>GSGDSGSPGIATPLVLGENLCSINGWVPTYRGEGTTGKIPDEQMLTRQNFVSCSDKECRRFFVSMGYGTTTNFADLIVSEQMNVYSVKLGDPPTPDKLKFEAVGWSASSCHDGFQWTVLSVAGDGFVSILYGGIITDTIHPTNGGPLRTQASSCICNDGTCYTIIADGTTYTASSHRLYRLVNGTSAGWKALDTTGFNFEFPTCYYTSGKVKCTGTNLWNDAKRPFLEFDQSFTYTFKEPCLGFLGDTPRGIDTTNYCDKTTTEGEGGIQGFMIEGSNSWIGRIINPGSKKGFEIYKFLGTLFSVQTVGNRNYQLLSNSTIGRSGLYQPAYESRDCQELCFWIEIAATTKAGLSSNDLITFCGTGGSMPDVNWG[4x]

We have characterized a new influenza virus from a flat-faced fruit bat (Artibeus planirostris) in the Amazon River basin in northern Peru. While our phylogenetic analysis indicated that the Peruvian bat virus shares common ancestry with recently identified Guatemalan H17N10 bat viruses, their genetic and phylogenetic divergence is such that we propose that their HA and NA genes be designated as new subtypes H18 and N11, respectively. The influenza HA and NA proteins are critical for interaction with the host and determining the subtype of influenza type A viruses. We determined crystal structures of the A/bat/Peru/10 HA and NAL proteins expressed in a baculovirus system.

The extensive sequence divergence of A/bat/Peru/10 NAL from the recently characterized N10 prompted us to determine its X-ray structure in two crystal forms at 2.68 Å and 3.0 Å. The N11 NAL forms a typical “box-shaped” tetramer, containing six four-stranded, antiparallel β-sheets in a propeller-like arrangement. Comparison of the A/bat/Peru/10 NAL monomer with other NA structures reveals surprising similarity despite low sequence identity (29.6%). In addition, a calcium required for stabilization of all known influenza A and B NA active sites is conserved in N11 NAL. Taken together, the N11 NAL and the N10 NAL are homologous proteins characterized by highly diverged putative active sites. Among the eight conserved charged and polar residues that interact with substrate in all other influenza A and B subtypes, only Arg118, Arg224, Glu276 are conserved (N2 numbering) as in N10 NALs. Arg292 and Arg371, critical for sialic acid binding, are replaced in A/bat/Peru/10 NAL by Thr and Lys, respectively. The N11 NAL active site pocket is much wider than other flu A and B NAs, including 1918 N1, due mainly to 150- and 430-loop movements. The glycerol moiety of a canonical sialic acid, as observed in other flu A and B NA structures, would clash with the N11 NAL active site. N11 NAL catalyzes extremely low levels of sialic acid cleavage as observed for N10 NAL, and similar to H18 HA, N11 NAL exhibited no binding to 610 diverse natural glycans including sialosides in a glycan microarray assay.> SNAILSLSYRGGRLIDSSGYGATMNVGSDVIFNDIGNGQFKLNNSENSNITAHQSKFVVYDSMFDNFSINFWVRTPKYNNNDIQTYLQNEYTIISCIKNDSGWKVSIKGNRIIWTLIDVNAKSKSIFFEYSIKDNISDYINKWFSITITNDRLGNANIYINGSLKKSEKILNLDRINSSNDIDFKLINCTDTTKFVWIKDFNIFGRELNATEVEERYKIQSSTNTLKDFWGNPLRYDTQYYL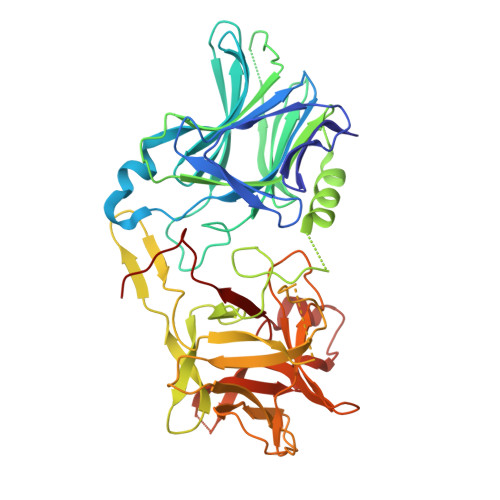FNQGMQNIYIKYFSKASMGETAPRTNFNNAAINYQNLYLGLRFIIKKASNSRNINNDNIVREGDYIYLNIDNISDESYRVYVLVNSKEIQTQLFLAPINDDPTFYDVLQIKKYYEKTTYNCQILCEKDTKTFGLFGIGKFVKDYGYVWDTYDNYFCISQWYLRRISENINKLRLGCNWQFIPVDEGWTELQ>[16x]MAGKPKLHYFNGRGRMEPIRWLLAAAGVEFEEKFIGSAEDLGKLRNDGSLMFQQVP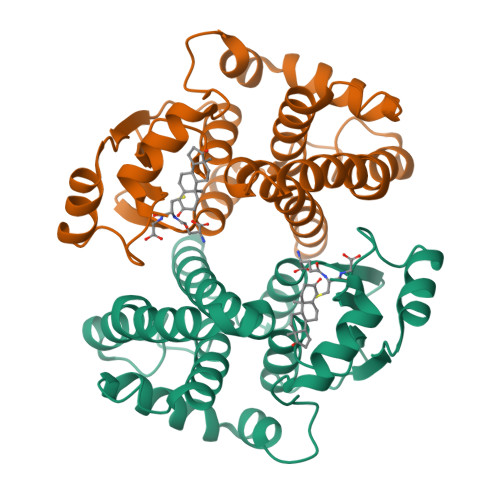MVEIDGMKLVQTRAILNYIASKYNLYGKDIKERALIDMYTEGMADLNEMILLLPLCRPEEKDAKIALIKEKTKSRYFPAFEKVLQSHGQDYLVGNKLSRADISLVELLYYVEELDSSLISNFPLLKALKTRISNLPTVKKFLQPGSPRKPPADAKALEEARKIFRF>[4x]GASKKSAAEASKKPRQKRTATKAYNVTQAFGRRGPEQTQGNFGDQELIR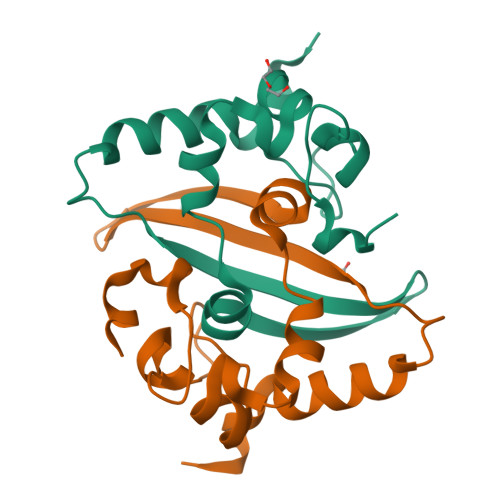QGTDYKHWPQIAQFAPSASAFFGMSRIGMEVTPSGTWLTYTGAIKLDDKDPNFKDQVILLNKHIDAYKTFP>MTGTVSRRKKIAMIGSGMIGGTMGYLCVLRELADVVLFDVVTGMPEGKALDDSQATSIAD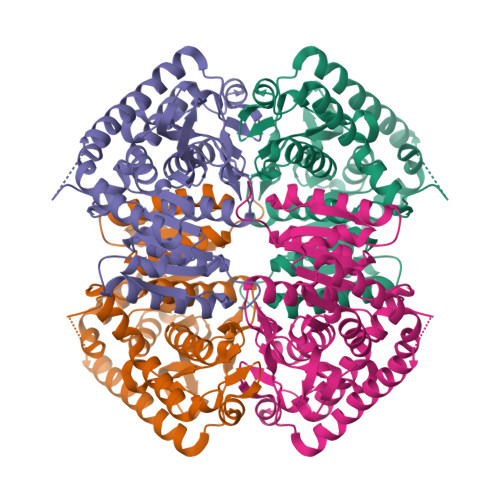TNVSVTSANQYEKIAGSDVVIITAGLTKVPGKSDKEWSRNDLLPFNAKIIREVAQGVKKYCPLAFVIVVTNPLDCMVKCFHEASGLPKNMVCGMANVLDSARFRRFIADQLEISPRDIQATVIGTHGDHMLPLARYVTVNGFPLREFIKKGKMTEAKLAEIVERTKKAGGEIVRLLGQGSAYYAPALSAITMAQAFLKDEKRVLPCSVYCQGEYGLHDMFIGLPAVIGGGGIEQVIELELTHEEQECFRKSVDDVVELNKSLAALGPG[2x]> GPGSMTLLMTQDELKRLVGEAAARYVTDNVPQGAVIGVGTGSTANCFIDALAAVKDRYRGAVSSSVATTERLKSHGIRV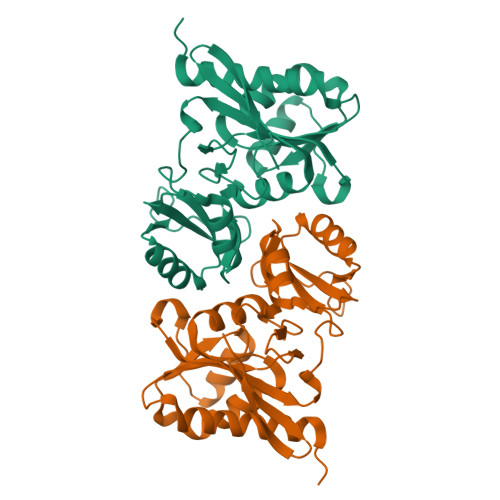FDLNEIESLQVYVDGADEIDESGAMIKGGGGALTREKIVASVAETFVCIADASKRVAMLGQFPLPVEVVPMARTAIGRRLAALGGVPVLRVKQDGTPYVTDNGNEILDVKGLRIDDPRALEAAINGWPGVVTVGLFAQRGADLCLLGTEHGVETLRYAAR>MRGSHHHHHHGSMPVAGSELPRRPLPPAAQERDAEPRPPHGELQYLGQIQHILRCGVRKDDRTGTGTLSVFGMQARYSLRDEFPLLTTKRVFWKGVLEELLWFIKGSTNAKELSSKGVKIWDANGSRDFLDSLGFSTREEGDLGPVYGFQWRHFGAEYRDMESDYSGQGVDQLQRVIDTIKTNPDDRRIIMCAWNPRDLPLMALPPCHALCQFYVVNSELSCQLYQRSGDMGLGVPFNIASYALLTYMIAHITGL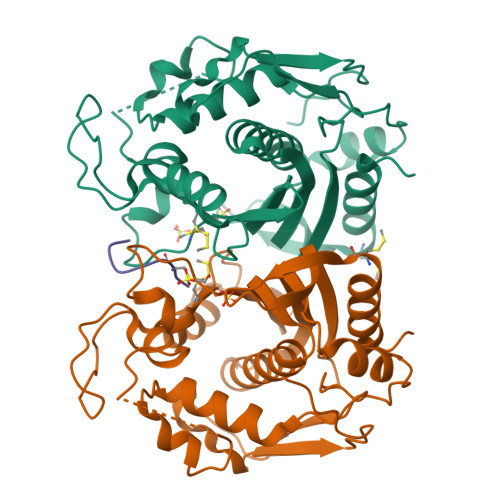KPGDFIHTLGDAHIYLNHIEPLKIQLQREPRPFPKLRILRKVEKIDDFKAEDFQIEGYNPHPTIKMEMAV[2x];> LSCQLYQR>MGPAFEFAVAMMKRNSSTVKTEYGEFTMLGIYDRWAVLPRHAKPGPTILMNDQEVGVLDAKELVDKDGANLELTLLKLNRNEKFRDIRGFLAKEEVEVNEAVLAINTSKFPNMYIPVGQVTEYGFLYLGGTPTKRMLMYNFPTRAGQCGGVLMSTGKVLGIHVGGNGHQGFS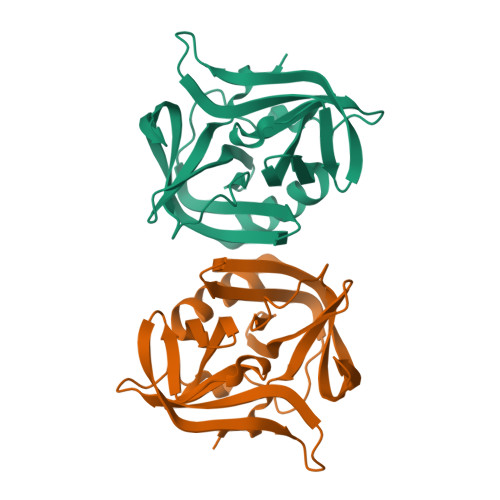AALLKHYFNDEQ[2x]>MHHHHHHAAACERALQYKLGDKIHGFTVNQVTSVPELFLTAVKLTHDDTGARYLHLAREDTNNLFSVQFRTTPMDSTGVPHILQHTVLCGSQKYPCRDPFFKMLNRSLSTFMNAFTASDYTLYPFSTQNPKDFQNLLSVYLDATFFPCLRELDFWQEGWRLEHENPSDPQTPLVFKGVVFNEMKGAFTDNERIFSQHLQNRLLPDHTYSVVSGGDPLCIPELTWEQLKQFHATHYHPSNARFFTYGNFPLEQHLKQIHEEALSKFQKIEPSTVVPAQTPWDKPREFQITCGPDSFATDPSKQTTVSVSFLLPDITDTFEAFTLSLLSSLLTSGPNSPFYKALIESGLGTDFSPDVGYNGYTREAYFSVGLQGIVEKDIETVRSLIDRTIDEVVEKGFEDDRIEALLHKIEIQMKHQSTSFGLMLTSYIASCWNHDGDPVELLKLGNQLAKFRQCLQENPKFLQEKVKQYFKNNQHKLTLSMRPDDKYHEKQAQVEATKLKQKVEALSPGDRQQIYEKGLELRSQQSKPQDASCLPALKVSDI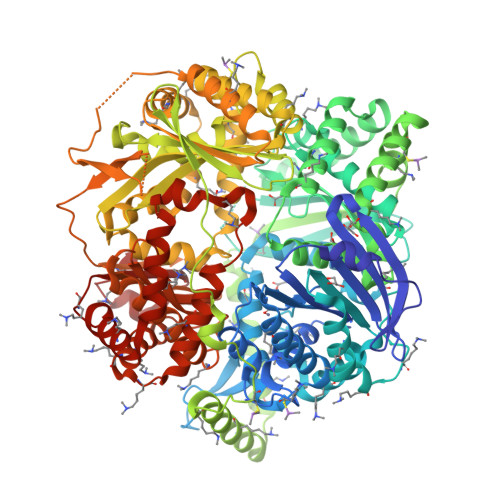EPTIPVTELDVVLTAGDIPVQYCAQPTNGMVYFRAFSSLNTLPEELRPYVPLFCSVLTKLGCGLLDYREQAQQIELKTGGMSASPHVLPDDSHMDTYEQGVLFSSLCLDRNLPDMMQLWSEIFNNPCFEEEEHFKVLVKMTAQELANGIPDSGHLYASIRAGRTLTPAGDLQETFSGMDQVRLMKRIAEMTDIKPILRKLPRIKKHLLNGDNMRCSVNATPQQMPQTEKAVEDFLRSIGRSKKERRPVRPHTVEKPVPSSSGGDAHVPHGSQVIRKLVMEPTFKPWQMKTHFLMPFPVNYVGECIRTVPYTDPDHASLKILARLMTAKFLHTEIREKGGAYGGGAKLSHNGIFTLYSYRDPNTIETLQSFGKAVDWAKSGKFTQQDIDEAKLSVFSTVDAPVAPSDKGMDHFLYGLSDEMKQAHREQLFAVSHDKLLAVSDRYLGTGKSTHGLAILGPENPKIAKDPSWIIR[2x]> MPLIFKIGYNVIPLQDVILPTPSSKVLKYLIQSGKLIPSLKDLITSRDKYKPIFISHLGFNQRRIFQTNGNLKTITKGSRLSSIIAFSTQANVLSEVADEGIFETVYGKFHIMIESIEIVEVEKLKEEVEKHMNDNIRVRFVSPTLLSSKVLLPPSLSERYKKIHAG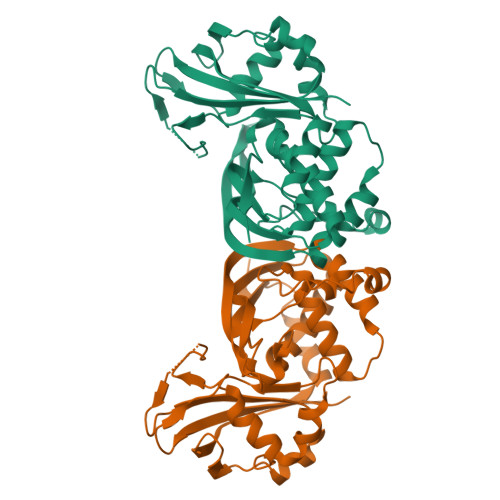YSTLPSVGLIVAYAYNVYCNLIGKKEVEVRAFKFGILSNALSRIIGYDLHPVTVAIGEDSKGNLRKARGVMGWIEFDIPDERLKRRALNYLLTSSYLGIGRSRGIGFGEIRLEFRKIEEKEG>KVTLPDLKWDFGALEPYISGQINELHYTKHHQTYVNGFNTAVDQFQELSDLLAKEPSPANARKMIAIQQNIKFHGGGFTNHCLFWENLAPESQGGGEPPTGALAKAIDEQFGSLDELIKLTNTKLAG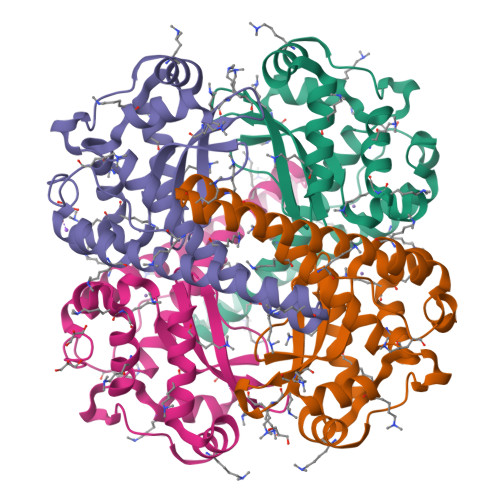VQGSGWAFIVKNLSNGGKLDVVQTYNQDTVTGPLVPLVAIDAWEHAYYLQYQNKKADYFKAIWNVVNWKEASRRFDAGKI[4x]>MRKIGIIGGTFDPPHYGHLLIANEVYHALNLEEVWFLPNQIPPHKQGRNITSVESRLQMLELATEAEEHFSICLEELSRKGPSYTYDTMLQLTKKYPDVQFHFIIGGDMVEYLPKWYNIEALLDLVTFVGVARPGYKLRTPYPITTVEIPEFAVS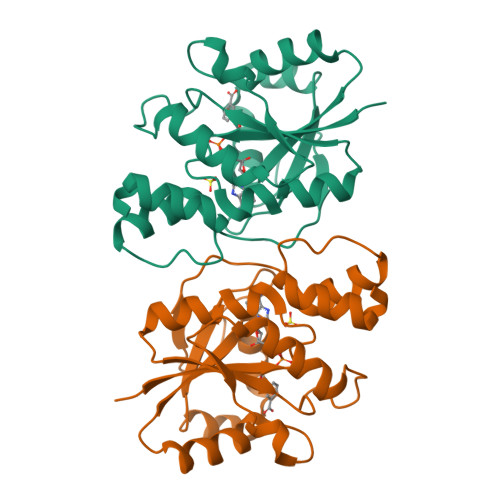SSLLRERYKEKKTCKYLLPEKVQVYIERNGLYES[3x]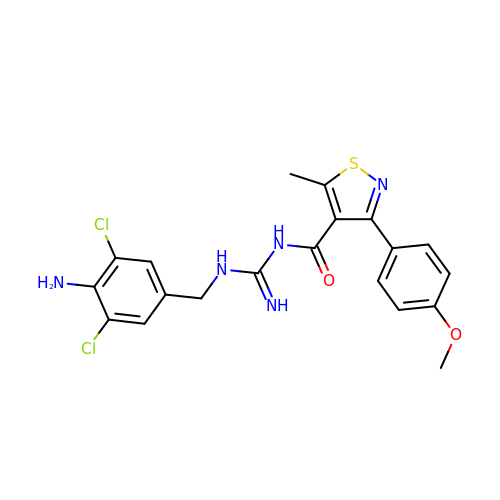N-[N-(4-amino-3,5-dichlorobenzyl)carbamimidoyl]-3-(4-methoxyphenyl)-5-methyl-1,2-thiazole-4-carboxamide | C20 H19 Cl2 N5 O2 S | DPJQBOWFYJTIJB-UHFFFAOYSA-N Herein, we have chosen to use an extracellular dye-type heme peroxidase found in Streptomyces lividans and referred to as DtpAa. The overall structure reveals a ferredoxin-like fold typical of dye decolourizing peroxidases with two DtpAa monomers in the crystallographic asymmetric unit. Heme enzymes catalyse many essential reactions in biology and understanding their structures throughout their reaction cycles is of high interest, prompting extensive efforts made to obtain ‘intact’ structures at high resolution. A major challenge is to obtain the higher valence states of these proteins, for example peroxidases (FeIII resting state and FeIV intermediate states), as these states are phenomenally sensitive to reduction in synchrotron experiments caused by the presence of large numbers of solvated electrons or other radiolytically produced species, generated by the interaction of X-rays with the crystal.

Serial synchrotron crystallography was carried out at Diamond Light Source beamline I24 at an X-ray energy of 12.8 keV using the same chip and translation system as used for SFX at SACLA. Following each translation of the chip to bring a fresh aperture/crystal into the beam, a series of 10 ms exposures were recorded using the PILATUS3 detector in shutterless mode. We first describe an MSS experiment series comprising five dose points with a dose increment of 32.8 kGy (MSS1). An increase in unit-cell volume and trends in scaling statistics clearly indicate the onset of global radiation damage resulting from disorder in the crystalline lattice as dose is accumulated. With increasing dose, distinct changes occur around the heme pocket consistent with reduction of the heme iron by X-ray generated solvated photoelectrons. A near-linear relationship is observed, demonstrating that water migration away from the Fe is dose-dependent under the conditions used. The elongation of the iron—water bond is consistent with FeIII to FeII reduction.

>GSAVPFHGAHQAGIATPVQDRLHFAAFDVTTEDRAAFVALLKEWTAAARRLTAGHAVGEGAYGGLPEAPPDDTGEALGLKPSRLTLTIGFGPSLFTRFGLADLRPEALADLPKFPGDNLDRARSGGDLCVQACADDPQVAVHAIRNLARIGFGKVVVRWSQLGFGKTSSTTPDKQTPRNLLGFKDGTRNIAGTEKDRLDRFVWAAEKDGTPWMTGGSYLVARRIRMHIETWDRASLQEQEDVFGRDKGEGAPVGKAKERDEPFLKAMKPDAHVRLAHPDSNGGATLLRRGYSFTDGTDGLGRLDAGLFFLAYQRDIRTGFVPVQRNLATDALNEYIQHVGSAVFAVPPGVRDADDWWGSTLF[2x]> MKLPYKLQDVYDGESQAKFTVISTFAGGGGSSTGYRLAGAKILCINEFVEEARKTYAANYPSTPIVPDDIKQLTGGDFLKITGLKPRELDILDGSPPCSAFSVAGSMCRGEGSKHSDGWGKTKNYSDGKKVENIEDLFFEFIRVAKGIQPKVIVAENVKGLTIGEAKTYYAKITNAFEDIGYLVTSKVMKSSHYGVGQARERLIFIAVRQDIADKVGLNILTVSSLFPPTSSEDTTIGDIIGGVEQDPEYIQSLVDHMTKSGIYKKVVSKM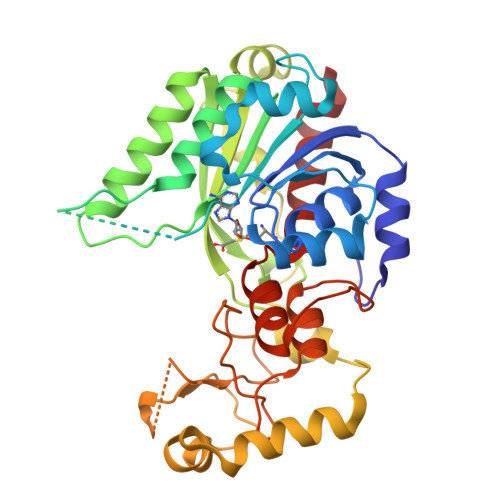PKNPKKILSGMDYHEKGHCFNTKRASFYKPSPTLTASGGLIHWNEDRVLSVPELKRIQSLPDDFILTGSHSQQTERVGRMVPPLMMKAIAENIYKEVLSKL>GSMAPRAGFDAEQVRDKARKDLLHLLEGVRGKKNLVIEKDLAGPLGVIVKASTLRDYGVDNFFFLENKNTGTSQRNIVFIARGESVRNAHAIAAQIKRIQRESQTSHDFHIFWVPRRTLFSDKVLEEAGVLGDANISELPLYFFPLERDVLSLELNDSFRDLYLAKDPTPVFLLSRALMGIQKKHGLFPRIIGKGENAKRVADLLSRMRQELLAGEEAGESDRAGLSPSTTIESVIIIDREVDFVTPLLTQLTYEGLIDEYFGIQNNQTDVDAVIVGAPAQSAASTSTAVPTNSSQSRKRKIQLDGSDSLYSQLRDANFAIVGSLLNTVARRLKSDYESRHNTKTTAELKEFVKKLPGYQAEQQSLKIHSNIAEEIINYTRTEIFNKLLEVQQNLAAGADPSSQFDSIEELVARDTPLPQVLRLLCLYSCISGGIKTKELDHFRRLVLQGYGHQHLLTLHNLERLQMFLSKSSPLASMITMSGSSGGPDQKTNYTYLRKQLRLIVDEVNEQDPNDIAYVYSGYAPLSIRLVQCVLQKQYLLSITKGSGTVIAAGPVAGGGAQGWKGFEEIVKHARGPTFDEIQKGEDKAVKARALLSGSSGDKKTVFVVFVGGITFTEIAALRFIAKQEEARRNIVICTTSIINGNRMMNAAIETATFEKTTVTTAAAQ[2x];>[2x]MGSSFEVIARTAYEEGRTRLATELLNHEPRAGRQVPLLLSMEEDELALDKAIESGDTDLIYFVIHQLRRKLPLASFFRVVSSRPTASAMVEALARNSDGDGNEDTALLKDLYYQDDRRLDGASVFIREALQQPETRTASDKLDLAANLLQGNQKEHVFELGALKEAKMLLRMQETFERDLT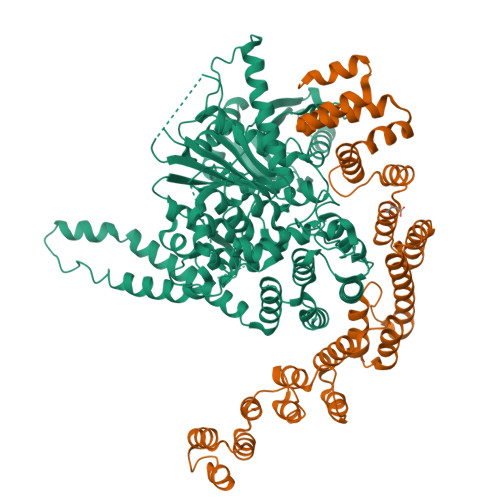DSFVGLSVNQTMFKLIKLGYHGRAKKIQSEFKVPERVAWWIRLQALVAKRDWNEIEEISRQRKSPIGWEPFFNQVLQAGNPRLAATFIPKCTNLEPGQTITMYEKCGMRVKAAEEAVRLKDTEAWNRLLEAAGRNTAEGREIERLGATVFKK> AMAISITCPPPMSVEHADIWVKSYSLYSRERYICNSGFKRKAGTSSLTECVLNKATNVAHWTTPSLKCIRDPALVHQRPAP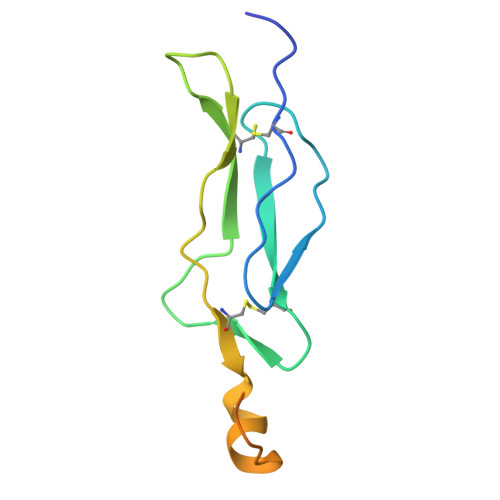PSTVTTAGVTPQPESLSPSGKEPAAS>[2x]SE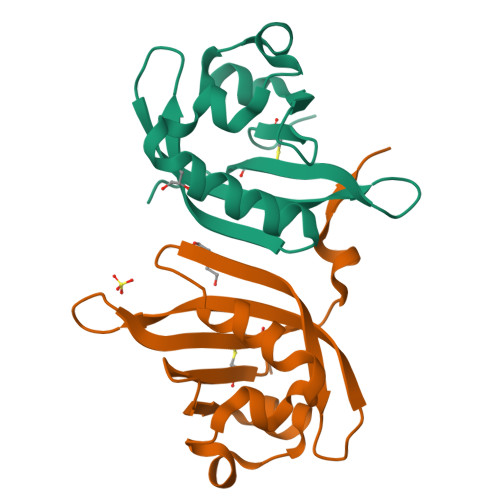FESQPCVSIDLRGNITSWNRAAEQLYQFKEGEVMGRNLVDLIVPPNAKTAALDTIMRVGQGEVWIGQFSCVRRDNAILNTVVTQKPILDDDQKISGISVCTEPYSMPELMARNY>[2x]MYVPGFGEASPEAKAAKHLHDFFTYVAVRIV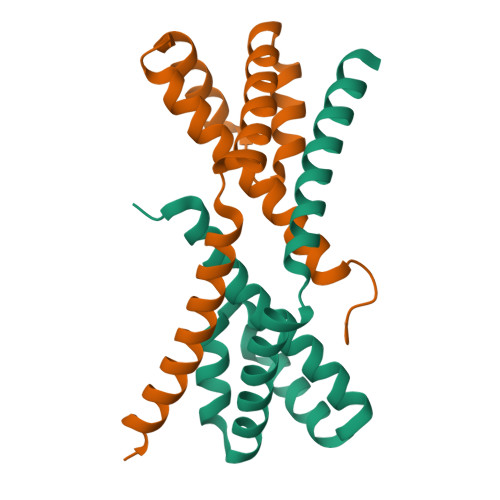SAQLESYNPEAYMELREFLDTNSVSDGDKFLATLMRRSSRHMNLALRILEVRSAYAKNDFEWDNMKRLAFKNVDDSNTRLMREYVLETSHVETDSDK The imidazole glycerol phosphate synthase from Thermotoga maritima forms a heterodimeric bienzyme complex consisting of the two subunits HisF and HisH (HisFH). The HisFH complex catalyzes the synthesis of the histidine precursor imidazole glycerol phosphate (ImGP) and the purine precursor 5-aminoimidazole-4-carboxamide ribonucleotide (AICAR) from N′-[(5′-phosphoribulosyl) formimino]-5-aminoimidazole-4-carboxamide ribonucleotide (PrFAR) and glutamine (Gln)9,10. This reaction takes place in two main steps and starts with the hydrolysis of Gln to glutamate (Glu) and ammonia in the glutaminase subunit HisH. The ammonia then migrates over 25 Å from the HisH active site through a central tunnel across the beta-strand barrel of HisF to the HisF cyclase active site at the opposite face of the barrel.

In order to visualize the structural changes that take place upon formation of the active conformation, we determined the crystal structure of HisFH in the presence of ProFAR and Gln. We used the inactive hC84A mutant for crystallization, which shows identical CSPs to the hC84S mutant and solved the structure of the complex to a resolution of 2.06 Å. The asymmetric unit contains three HisFH complexes, all of which show electron density for Gln. Two of the complexes (chains A/B and C/D) adopt a conformation highly similar to previously published apo structures of the HisFH complex. In one of these HisFH complexes in the inactive conformation (chains A/B) the HisF active site shows unambiguous electron density for a ProFAR molecule. In contrast, the third HisFH complex (chains E/F) in our crystal shows electron density for both ligands and large, long range conformational changes that extend between both active sites. First, the β1α1 loop (fL1) in HisF moves by 25 Å from a position close to helix fα1 to a state, in which it covers the HisF active site (red arrow). In the closed state fL1 forms a short beta sheet and several highly conserved residues in the loop make extensive contacts with ProFAR and the HisF active site residues: fK19 forms a salt bridge with fD176 and the phosphate of ProFAR, the aromatic side chain of fF23 forms a π-stacking interaction with the imidazole ring of ProFAR and fN22 forms hydrogen bonds to the backbone carbonyls of fI173/fD174/fD176. Third, the formation of the active conformation is accompanied by an inter-subunit reorientation of the complex, similar as described in a previously reported hyperactive HisFH variant containing an unnatural amino acid at the subunit interface. This can, e.g., be visualized through the angle between the Cα atoms of fF120, hW123, and hG52 which is reduced from 25° in the inactive conformation to 10° in the active conformation. As a result, the amide group of the substrate Gln in the active site rotates into the newly formed oxyanion hole and forms hydrogen bonds with hV51/hL85 (through its amide carbonyl group) and hH178/hV140 (through its amide NH2 group).

>[3x]MLAKRIIACLDVKDGRVVKGTNFENLRDSGDPVELGKFYSEIGIDELVFLDITASVEKRKTMLELVEKVAEQIDIPFTVGGGIHDFETASELILRGADKVSINTAAVENPSLITQIAQTFGSQAVVVAIDAKRVDGEFMVFTYSGKKNTGILLRDWVVEVEKRGAGEILLTSIDRDGTKSGYDTEMIRFVRPLTTLPIIASGGAGKMEHFLEAFLAGADAALAASVFHFREIDVRELKEYLKKHGVNVRLEGL;>[3x]MGMRIGIISVGPGNIMNLYRGVKRASENFEDVSIELVESPRNDLYDLLFIPGVGHFGEGMRRLRENDLIDFVRKHVEDERYVVGVALGMQLLFEESEEAPGVKGLSLIEGNVVKLRSRRLPHMGWNEVIFKDTFPNGYYYFVHTYRAVCEEEHVLGTTEYDGEIFPSAVRKGRILGFQFHPEKSSKIGRKLLEKVIECSLSRR> MENTENSVDSKSIKNLEPKIIHGSESMDSGISLDNSYKMDYPEMGLCIIINNKNFHKSTGMTSRSGTDVDAANLRETFRNLKYEVRNKNDLTREEIVELMRDVSKEDHSKRSSFVC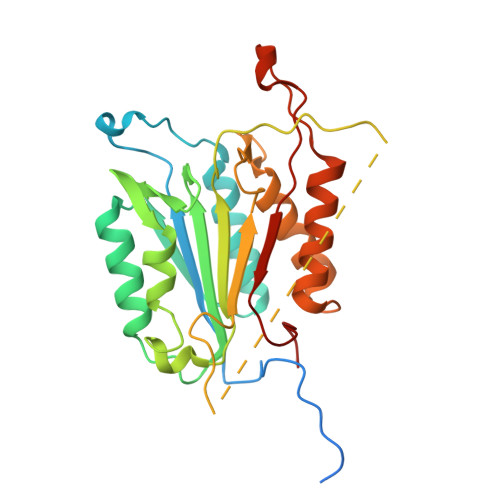VLLSHGEEGIIFGTNGPVDLKKITNFFRGDRCRSLTGKPKLFIIQACRGTELDCGIETDSGVDDDMACHKIPVEADFLYAYSTAPGYYSWRNSKDGSWFIQSLCAMLKQYADKLEFMHILTRVNRKVATEFESFSFDATFHAKKQIPCIQSMLTKELYFYH> MAKQYDDNECPFCDEVSKYEKLAKIGQGTFGEVFKARHRKTGQRVALKKVLMENEKEGFPITALREIKILQLLKHENVVNLIEICRTKASPYNRCKGSIYLVFDFCEHDLAGLLSNVLVKFTLSEIKRVMQMLLNGLFYIHRNKILHRDMKAANVLITRDGVLKLADFGLARAFSLAKNSQPNRYTNRVVTLWYRPPELLLGERDYGPPIDLWGAGCIMAEMWTRSPIMQGNTEQHQLALISQLCGSITPEVWPNVDNYELYEKLELVKGQKRKVKDRLAAYVRDPYALDLIDKLLVLDPAQRIDSEDALEHDFFWSDPMPSDLKGMLST;> MEGERKNNNKRWYFTREQLENSPSRAFGVDPDKELSYRQQAANLLQDMGQRLNVSQLTINTAIVYMHRFYMIQSFTRFPGNSVAPAALFLAAKVEGQPKKLEHVIRVAHTCLHPQESLPDTRSEAYLQQVQDLVILESIILQTLGFELTIDHPHTHVVKCTQLVRASKDLAQTSYFMATNSLHLTTFSLQYTPPVVACVCIHLACKWSNWEIPVSTDGKHWWEYVDATVTLELLDELTHELLQILEKTPNRLKRIWNWR

Cyclin-dependent kinase 9 (CDK9) has emerged as an attractive CDK target owing to its role in potentiating oncogenic transcription programs. CDK9 is a transcription-regulating CDK that acts as a subunit of the positive transcription elongation factor b (P-TEFb). P-TEFb is recruited to the genome by transcription factors and other components of the transcription machinery, where it is sequestered in an inactive ribonucleotide protein complex (7SK snRNP). Its activation is facilitated through multiple molecular mechanisms, including recruitment of specific transcription factors such as MYC, transcription elongation-promoting complexes such as those including bromodomain-containing protein 4 (BRD4) and the super elongation complex (SEC), and by splicing factors and co-transcriptional RNA processing events. Activated CDK9 within the P-TEFb complex phosphorylates multiple transcription substrates—most notably the serine 2 (Ser2) residue of the carboxy-terminal domain (CTD) heptad repeats of RNA polymerase II (RNAP II). CDK9 releases this paused state by phosphorylating the RNAP II Ser2 and allowing transcriptional elongation to proceed, making CDK9 an attractive target to attenuate unchecked transcriptional addiction to deregulated MYC. Phosphorylation of RNAP II Ser2 is an evolutionarily conserved and rate-limiting requirement for productive transcription elongation and mRNA processing. Although CDK9 is an essential gene and broadly required for global transcription, multiple studies have implicated highly transcribed, short half-life genes such as MYC and MCL1 as being uniquely sensitive to CDK9 inhibition.

Herein we report a medicinal chemistry effort to optimize this hit, prioritizing maintenance of CDK9 selectivity while improving the on-target potency and overall physicochemical and pharmacokinetic (PK) properties. This allowed us to advance the initial SMM hit to the potent, selective, orally bioavailable CDK9 inhibitor 28 (KB-0742). Co-crystallization of compound 28 with CDK9/cyclin T1 confirmed ligand binding as predicted in our model, albeit at 3.8 Å resolution. Regardless of the low resolution, the co-crystal structure provided a partial density to confirm our predicted binding mode of compound 28. In brief, the amino-pyrazolopyrimidine core of 28 aligns to hinge Cys106 of the ATP-competitive binding pocket as postulated; the terminal amine of the diamino-cyclopentane moiety interacts with Asp109 in a HBD manner; and the 3-pentyl group points to a hydrophobic patch formed by the Leu156 side chain. An additional methyl to make symmetric 3-pentyl 28 delivered a 6 nM compound. A subsequent CDK selectivity panel demonstrated that this compound possessed a ≥66-fold selectivity toward CDK9 compared to others tested.> MDLTNGGVSPAATSAPLDWTTFRRVFLIDDAWRPLMEPELANPLTAHLLAEYNRRCQTEEVLPPREDVFSWTRYCTPDEVRVVIIGQDPYHHPGQAHGLAFSVRANVPPPPSLRNVLAAVKNCYPEARMSGHGCLEKWARDGVLLLNTTLTV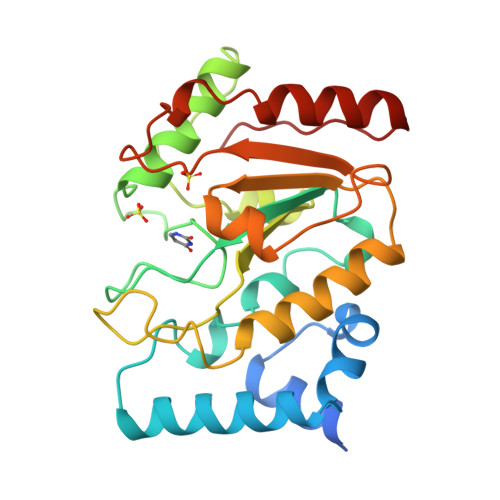KRGAAASHSRIGWDRFVGGVIRRLAARRPGLVFMLWGTHAQNAIRPDPRVHCVLKFSHPSPLSKVPFGTCQHFLVANRYLETRSISPIDWSV> GMIPLKIAIAGANGRMGRVLVEAVNNHPDTVLSGALEHSGSEALGLDAGYAVGLKTGIAISDDVDAVLAQSDVLIDFTRPEPTLKHLQKCVEKQVNIIIGTTGFDDAGKAAIRAAAEKTGIVFAANFSVGV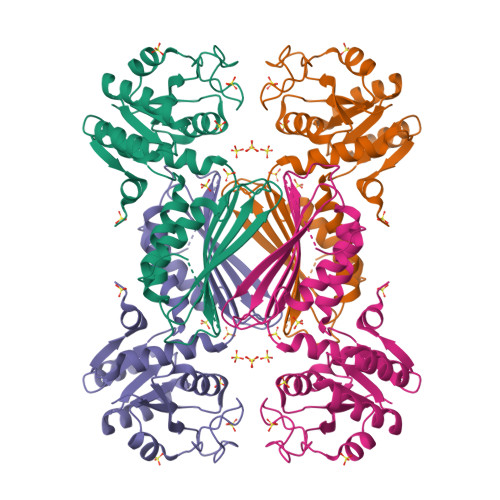NLTFHILDTVARVLNEGYDIEIIEGHHRHKVDAPSGTALRMGEVIAGALGRDLKQCAVYGREGHTGPRDPSTIGFATVRAGDIVGDHTALFATDGERVEITHKAGSRMTFAAGAVRAAVWVNGKTGLYDMQDVLGLNNR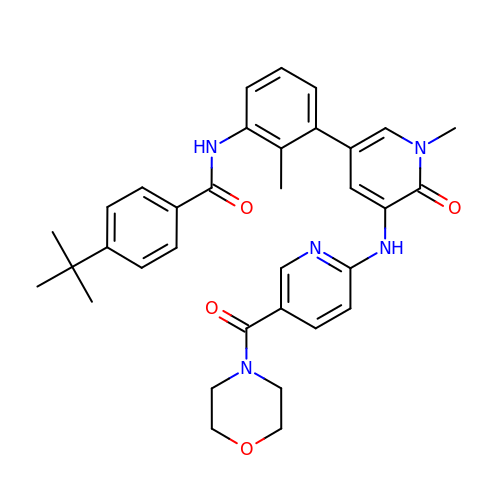4-tert-butyl-N-[2-methyl-3-(1-methyl-5-{[5-(morpholine-4-carbonyl)pyridin-2-yl]amino}-6-oxo-1,6-dihydropyridin-3-yl)phenyl]benzamide | C34 H37 N5 O4 | WHRCWROQSJHEBV-UHFFFAOYSA-N> MADKKTDIPTLIADSTKASLQDFNHDYGKQWTFGENWSNVNTMFETYVNKYLFPKINETLLIDIALGNRFNWLAKEQDFIGQYSEEYVIMDTIPIEMNLSKSEELMLKRNYPQMATRLYGSGIVKKQKFTLNNNDVRFNFQTLGDATNYALGVLRKKISDINVQEEKEIRAMMVDYAINQLQDSNRRTASSKEDLTERVFEAILNMQNNSAKYNEVHKASGGSVGQYTTVSKLSDIAILTTDSLKSYLLDTKIANTFQMAGIDFTDHIISFDDLGGVYKTTKDVTLANEDTINYLRAFGDYQAMIGDVIPTGSVFTFNVSDLKEFKGNIEEIKPQGELFAFIFDINALKYKRNTKGMLKEPFYNGEFDEVTHWIHYYSFKAMSPF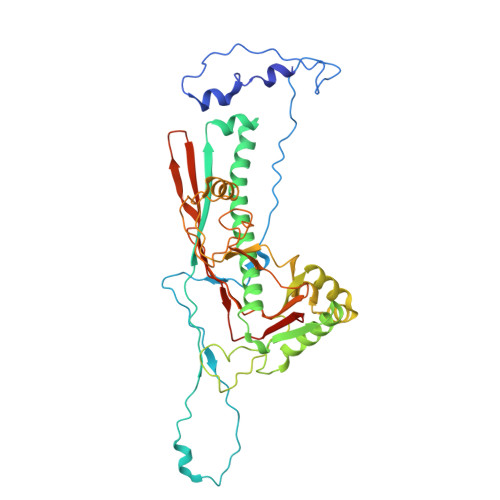FNKILITEAPKEQPDAGATE>MQEKSITIATEGGYAPWNFSGPGGKLDGFEIDLANALCEKMKAKCQIVAQNWDGIMPSLTGKKYDAIMAAMSVTPKRQEVIGFSIPYAAGINGFAVMGDSKLAEMPGLGETYSLDSQADAAKKAIADISSFLNGTTVGVQGSTTASTFLDKYFKGSVDIKEYKSVEEHNLDLTSGRLDAVLANATVLAAAIEKPEMKGAKLVGPLFSGGEFGVVAVGLRKEDTALKADFDAAIKAASEDGTIKTLSLKWFKVDVTPQHH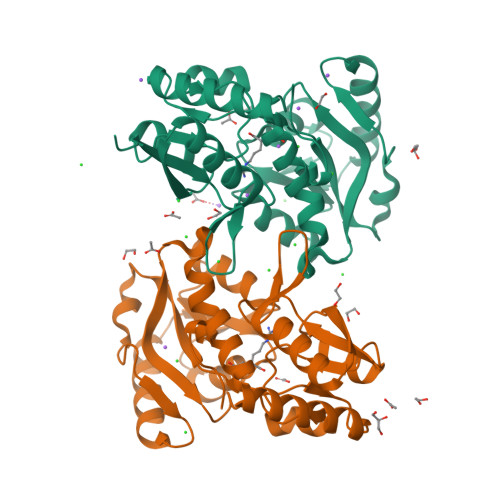HHHH[2x]> MVLTQQFVISNADLGRGHVVEALHPSSPLIALAGSKGRVLILNKTGKVEHQLPMQNVVAMEWECSTDTLAIITSSSSDVHLYTHRTRQTDTIDTKLKDLCFVCWSQSQPLFAIGSKSGQFVLYNRRTLRLVPVADTHKQRLISGMWVPAQDSRLLIISEDPSLSISDAEGKVLTTIPLPSVPKSVCVSGMANSPKSSSFAAVNLDNTLLIVDLRSYATAAGQFNSALGQITCLTAGINGEFLAGFASGTVALLDLAGSEVRLRGSLRLLKNAVEMVNFGEGSGVVAAVADNRVGLLRITEDGIAPTGDEASLESERGVPDLLAWSRDGQQLFVGTNQGNVTVFTLKVLNVSASYGTLVFSFTSNRTIGVKNLQDNRVVCTVPVNSDPAFISAGMAMLAAGVNNQVSYYEYFIPNSLPYPMVDPAKNVSQSSQQAHSVFLRTVEYPSPVTDLKVNSNLAAVVYDGRVQLSPIRDTPEAAAPVYFPESGDTRLVSIALSEVFFLYATTSRVSVYALHNLQQVATFTCNTGLKRAFANPACTRVAYVDDSSELFNVNLVTEVANKAEGYDPDQKMVLWDQAEATVFITYDSEKCATFVNTPHSRHGATCESVLVKDSSEDNLYTPLPPGYTPVTLFRGTVVCQTPNGTLETVPLQTHNNIFLRTPNAEAFYNNFSLNRLRWSSNNITSPQEAEDLAVKSLHMLDVELAIRVYRQLSQPSLVLCLEKIRHIHEKNLLLGHVSMIMGYMKDAQNFFLRSSQPLRALEMRRDMMQWERALTLAEQLAPEEVPIISRDYAQHLEYRGVYAKALEMYQKGLRQLPTGHASTELSVTVQEVERHNEQCRQGAARSQIRIGNIADAMKTVKESSEVSFVKECAKLCEENQKHE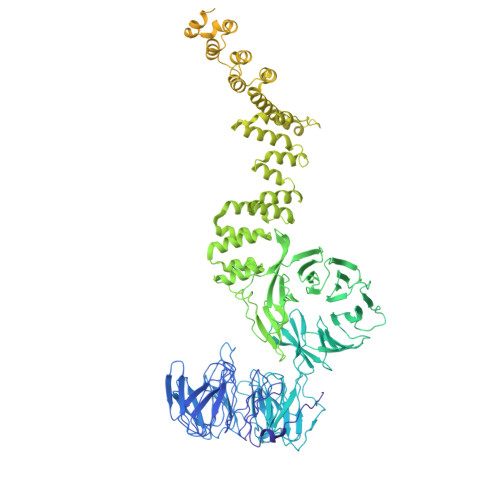EAAQLYEKAGDIERAATIYIERCKNLKAAERLLPFIKSRNIIGIYARGKEAEGAFVEAEKAFAQAEDWDNAVRLRIEKLNDLHGAYVIVRQTRSANAAALVAKKCTAQKEYGTAVEFLVLAKSLDEAFELAKTHDCMFNFESALLNQVQLKDGIAPLSNQADFTMIAEYYDNDGKAGQAGMYYHISGHYAKALNKYLESGQPEDIEKAVEVVGKAHSDSLTNKFIDYLMGETDGEPKDPSYIFKLYLAMGSYEKAAKTSVIISAKEQEIGNYKSAHKTLVEAYRILQQRNMHVSNDLRRALMLLHSYIIVKDLLKIMKDDDTACRMLLRVSRNIQKFPKHITTIVTTTVLQCLKSNFKKSAFEYACYLIQNEKHRAEMTEKSRKKIEGIVRRHSKDDAVDPVEPMLPCPYCDAPVAETELDCGACKNTIPFCIVTGKHIVKSDYTSTPCCGFPAIYSALMTRLSGTLTCPMCEATIDISNVNRETNPELKALL Lipoate protein ligases (Lpls) are responsible for the metabolism of lipoic acid. Specific enzymes catalyze the covalent attachment of lipoic acid to the acyltransferase (E2) subunit or H protein of the glycine cleavage system (GcvH) via an amide linkage between the ε-amino group of a specific lysine residue of these proteins and the lipoic acid carboxyl group. Here, a new lipoate protein ligase from M. hyopneumoniae was verified, and its structure was solved. Mhp-Lpl is composed of a large N-terminal domain (residues 1–254), a small C-terminal domain (residues 260–344), and a short polypeptide (residues 255–259) between the two domains.

To clearly see the interaction between Mhp-Lpl and lipoic acid, Mhp-Lpl was first reacted with ATP and lipoic acid and then crystallized after further purification. Lipoyl-AMP could be modeled into the density, despite its partial occupancy. The AMP part of lipoyl-AMP forms extensive hydrophobic interactions with the surrounding residues, including I80, L82, K138, L158, I166, L170, and V189. Among these residues, K138 forms an additional hydrogen bond with the carbonyl oxygen of lipoyl-AMP and plays essential roles in both lipoate adenylation and lipoate transfer reactions as shown in E. coli LplA. The aliphatic moiety of lipoic acid is enclosed in a hydrophobic tunnel formed by residues L20, Y40, T75, C90, A143, and Y152. Structural superposition revealed several key differences at the ligand binding sites between Mhp-Lpl and LplA molecules from other species. The residues corresponding to residue Q47 in Mhp-Lpl all have a small side chain, such as isoleucine or valine, in the LplA proteins from other species. The large-sized side chain of residue Q47 in Mhp-Lpl pushes the dithiolane ring of the lipoyl moiety away and flips toward the large β-sheet in the N-terminal domain. Correspondingly, the otherwise conserved histidine residue in LplA from other species at position 154 is replaced by a glycine residue in Mhp-Lpl, which enables the encapsulation of the dithiolane ring of the lipoyl moiety. Moreover, the conserved valine residue in the lipoate-binding loop (77 in Ec-LplA and 75 in Ef-LplA-2) is substituted with an isoleucine residue (I80), which enhances the hydrophobic interaction with lipoyl-AMP and explains why it is difficult to remove the unidentified AMP-fatty acid conjugate from Mhp-Lpl expressed in E. coli.

>[2x]MYLIEPKRNGKWVFDGAILLAIQYWAIKNLKLDETIVFPYICDPHVQIGYFQNPSVEVNLELLKQKNIEVVRRDTGGGAIYLDRNGVNFCFSFPYEKNKNLLGNYAQFYDPVIKVLQNIGIKNVQFSGKNDLQIEGKKVSGAAMSLVNDRIYAGFSLLYDVDFDFIGKILTPNQKKIEAKGIKSVSQRVTNLKNKLSKEYQNFSIFEIKDLFLTEFLKVNSVEKFKKYELTDSDWVQIDKMVAEKYKNWDFVWGLSPNYSFNRSIRTKVGTITFSLEINEGKISKIKISGDFFPKKSLLELENFLMGTKLTQDQLLNRLKDAKLEDYFSQKIDEEEICNLLLNLEHHHHHH>EELSVAQKQYVTAHGRQLVGQGATTLCTMKKLLDGVNSRVDTFEQQILTFVNNANANFRKISDDKVMAASLSASRLQEMQYMKSLGNSIIKYMGETGKRAKAAAAAASAALDEVLKWHCVDRTESHESSYSSTPNANCEPNAYKRDYYYEHSRLDPHKYSILCNYKVVSSTTTQTTFSNMERALEIWNQVKPKPYHMRVMICGAGAPAHQAAPAGRPCTVLENWLWNYRVTAHLIAKLEKDATLALRVMRYSEKVLEGDKESLAQHEERRKAAEARAAEEEAKRQAAEKAAEEARKALEEAEARRVAAEEQAEARRLEAEKAEKAKEAGQPVSEEKK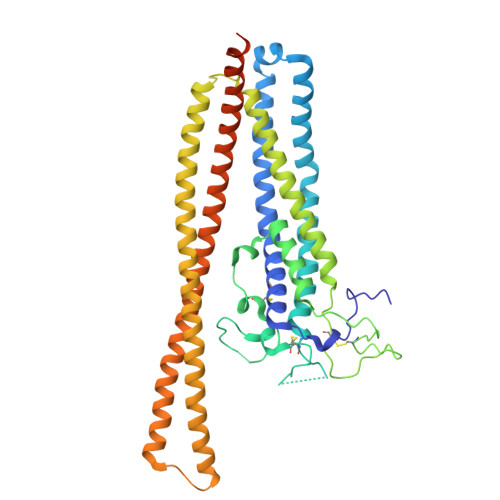KMLLEAVEKAEATEKAAEKQAKDSRKAFEEAEEERVKATEDAEAAKEEKKDAEESEEKLKKDVEKLAEELKEESKESGEEDDVNADHDDGGSEAKSGWIGTTK[2x]> MSKFGRKVPSNAKSQHNFSVIPSANIQRSVFNRSSGYKTTFDAGYLIPVFLDEALPGDTFHLKTSVLARLSTPVVPFMDNLRLDIQYFSVPYRLVWDNWQKFNGEQKNPGDSTDYLIPQIKAPAGGFPVGSLADYFGVPTGVENISVSALPFRAYNLIYNEWYRDENLINSAPLPLGDEEETGLANFPLRKRAKRHDYFTSALPWPQKGEGVEIGLGVPPSYTLEYPYYKEGMGFISSNYGASGNIGRTFPTYIARSSVGDDSSSNIGNAAYFSEGLENGINFPNAPARGRYDVLGGFDPNTPPVTLKKEGGEVVDNLTINSLRQAFQLQRLLERDARGGTRYIEIIRSHFGVISPDARVQRPEYLGSGSFDININPVLQNSATTDASPQGNLAAYGVSGGVNRGFSHSFVEHCFVIGLVSVRADLTYQQGIPRMFSRQTRFDFYWPALAHLGEQAILNKEIYAQGNAKDDEVFGYQERYAEYRYRPSQITGKLRSTDPQSLDVWHLAQRFDSLPALNQEFIEENPPM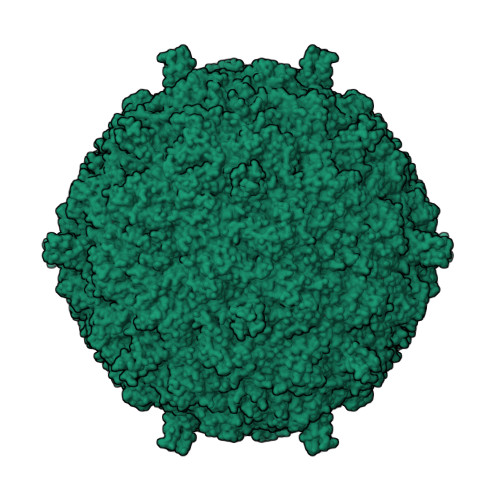KRVLAVQDEPQFIMDAFFDLKCVRPMPVYSVPGLIDHF;> MARSRRRMSKRSSRRSFRKYAKTHKRNFKARSMRGGIRL>[2x]VLEEDREPDFIEVTSLQEFKDIMSMDILTVACFWAD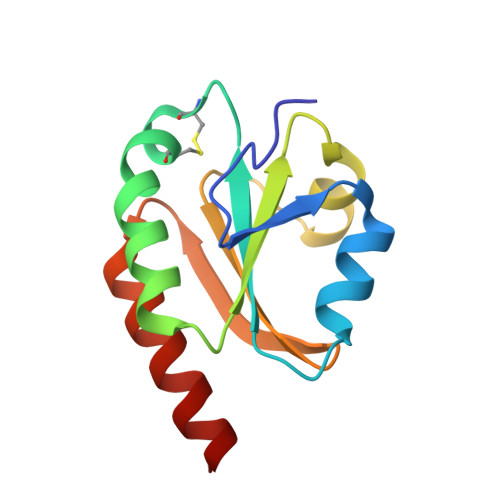DCGPCKLIEEPLKKIAEDFPDVVFALVDADKNPEIIKELNVKSLPTWIIARSGEYLGDVVGAKPDLLIEKIKNIKKNLEH> KEENNFINLYTVKNPLKCKIVDKINLVRPNSPNEVYHLEINHNGLFKYLEGHTCGIIPYYNELDNNPNNQINKDHNIINTTNHTN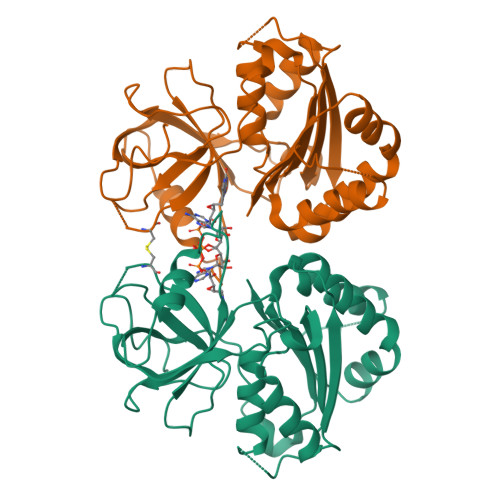HNNIALSHIKKQRCARLYSISSSNNMENLSVAIKIHKYEQTENAPNITNYGYCSGFIKNLKINDDIYLTGAHGYFNLPNDAIQKNTNFIFIATGTGISPYISFLKKLFAYDKNNLYNRNSNYTGYITIYYGVYNEDSILYLNELEYFQKMYPNNINIHYVFSYKQNSDATSFYVQDEIYKRKTEFLNLFNNYKCELYICGLKSIRYKVMDILKSHDQFDEKKKKRVHVEVY>[4x]GUGGUGAAGUCGCGG;>C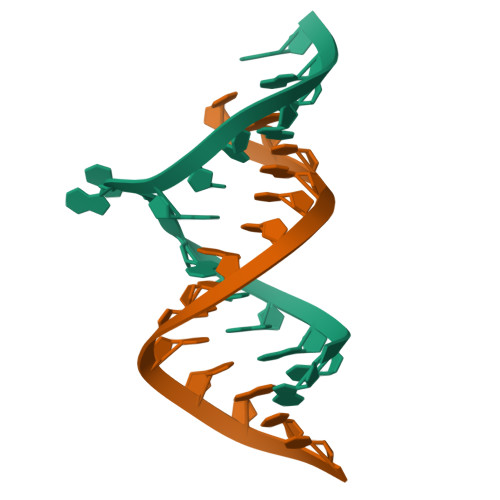GCGUCACACCACC[4x]>MDSFNPTTKTQAALTAALQAASTAGNPEIRPAHLLMALLTQNDGIAAPLLEAVGVEPATVRAETQRLLDRLPQATGASTQPQLSRESLAAITTAQQLATELDDEYVSTEHVMVGLATGDSDVAKLLTGHGASPQALREAFVKVRGSARVTSPEPEATYQALQKYSTDLTARAREGKLDPVIGRDNEIRRVVQVLSRRTKNNPVLIGEPGVGKTAIVEGLAQRIVAGDVPESLRDKTIVALDLGSMVAGSKYRGEFEERLKAVLDDIKNSAGQIITFIDELHTIVGAGATGEGAMDAGNMIKPMLARGELRLVGATTLDEYRKHIEKDAALERRFQQVYVGEPSVEDTIGILRGLKDRYEVHHGVRITDSALVAAATLSDRYITARFLPDKAIDLVDEAASRLRMEIDSRPVEIDEVERLVRRLEIEEMALSKEEDEASAERLAKLRSELADQKEKLAELTTRWQNEKNAIEIVRDLKEQLEALRGESERAERDGDLAKAAELRYGRIPEVEKKLDAALPQAQAREQVMLKEEVGPDDIADVVSAWTGIPAGRLLEGET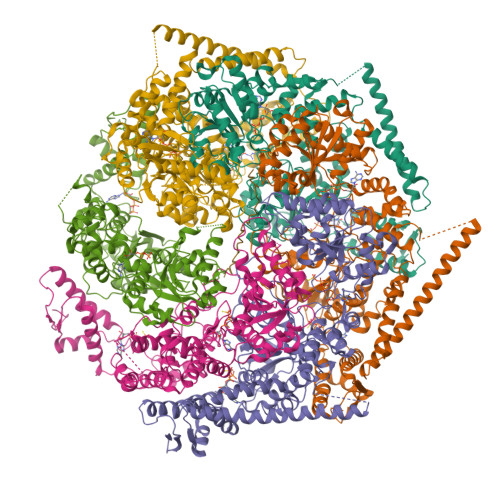AKLLRMEDELGKRVIGQKAAVTAVSDAVRRSRAGVSDPNRPTGAFMFLGPTGVGKTELAKALADFLFDDERAMVRIDMSEYGEKHTVARLIGAPPGYVGYEAGGQLTEAVRRRPYTVVLFDEIEKAHPDVFDVLLQVLDEGRLTDGHGRTVDFRNTILILTSNLGSGGSAEQVLAAVRATFKPEFINRLDDVLIFEGLNPEELVRIVDIQLAQLGKRLAQRRLQLQVSLPAKRWLAQRGFDPVYGARPLRRLVQQAIGDQLAKMLLAGQVHDGDTVPVNVSPDADSLILG[6x]>[2x]GSHPFDQAVVKD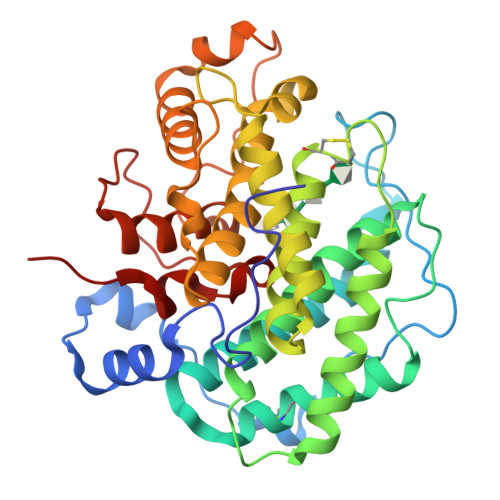PTASYVDVKARRTFLQSGQLDDRLKAALPKEYDCTTEATPNPQQGEMVIPRRYLSGNHGPVNPDYEPVVTLYRDFEKISATLGNLYVATGKPVYATCLLNMLDKWAKADALLNYDPKSQSWYQVEWSAATAAFALSTMMAEPNVDTAQRERVVKWLNRVARHQTSFPGGDTSCCNNHSYWRGQEATIIGVISKDDELFRWGLGRYVQAMGLINEDGSFVHEMTRHEQSLHFQNYAMLPLTMIAETASRQGIDLYAYKENGRDIHSARKFVFAAVKNPDLIKKYASEPQDTRAFKPGRGDLNWIEYQRARFGFADELGFMTVPIFDPRTGGSATLLAYKPQG>SMNTLSAIGDILHPLLHKNTSDLYELRYSSSFTGQELFMA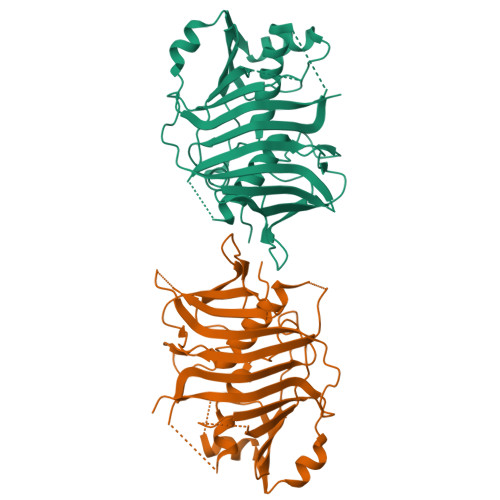DHLGNGQRFFPLIAYLEMARAAVKQAAGERAGTLSGIRMSHVATDDPLLVGDDLVQVHVGIYPEDTGELAYKIYSESNEDDTRSVVHSHGMVEFTSFVEVPTLDLPALQAESSEILTARQCYELLKERGMADHSEFQGIDQVYRAPGHVLVKLSLPSITMETAEQLVFHPSLLESLLPSTRYLITEATSPDSIRSIQLDGTFTLEELEIYENHPAVKYALIRFSDNVQAENETATLDIELCDEAGRIGIRMRGFSMGSEKRGATVGTTMLTPVWNAVSVEKG[2x]>[8x]MHHHHHHLVPRGSHMSVVGTPKSAEQIQQEWDTNPRWKDVTRTYSAEDVVALQGSVVEEHTLA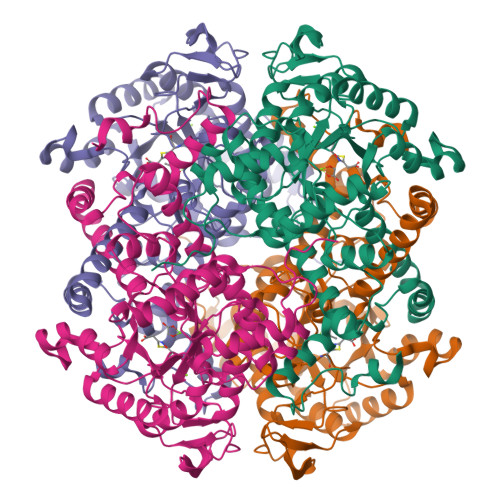RRGAEVLWEQLHDLEWVNALGALTGNMAVQQVRAGLKAIYLSGWQVAGDANLSGHTYPDQSLYPANSVPQVVRRINNALQRADQIAKIEGDTSVENWLAPIVADGEAGFGGALNVYELQKALIAAGVAGSHWEDQLASEKKXGHLGGKVLIPTQQHIRTLTSARLAADVADVPTVVIARTDAEAATLITSDVDERDQPFITGERTREGFYRTKNGIEPCIARAKAYAPFADLIWMETGTPDLEAARQFSEAVKAEYPDQMLAYNCSPSFNWKKHLDDATIAKFQKELAAMGFKFQFITLAGFHALNYSMFDLAYGYAQNQMSAYVELQEREFAAEERGYTATKHQREVGAGYFDRIATTVDPNSSTTALTGSTEEGQFH> EFGSMEFVNKQFNYKDPVNGVDIAYIKIPNAGQMQPVKAFKIHNKIWVIPERDTFTNPEEGDLNPPPEAKQVPVSYYDSTYLSTDNEKDNYLKGVTKLFERIYSTDLGRMLLTSIVRGIPFWGGSTIDTELKVIDTNCINVIQPDGSYRSEELNLVIIGPSADIIQFECKSFGHEVLNLTRNGYGSTQYIRFSPDFTFGFEESLEVDTNPLLGAGKFATDPAVTLAHELIHAGHRLYGIAINPNRVFKVNTNAYYEMSGLEVSFEELRTFGGHDAKFIDSLQENEFR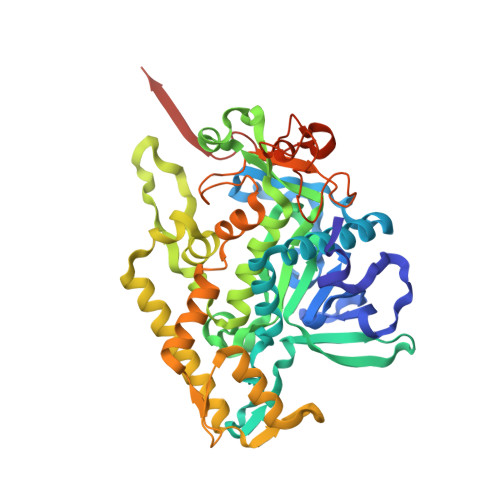LYYYNKFKDIASTLNKAKSIVGTTASLQYMKNVFKEKYLLSEDTSGKFSVDKLKFDKLYKMLTEIYTEDNFVKFFKVLNRKTYLNFDKAVFKINIVPKVNYTIYDGFNLRNTNLAANFNGQNTEINNMNFTKLKNFTGLFEFYKLLCVDGIITSKTKSLIEGR RET receptor tyrosine kinase plays vital developmental and neuroprotective roles in metazoans. GDNF family ligands (GFLs) when bound to cognate GFRα co-receptors recognize and activate RET stimulating its cytoplasmic kinase function. The bipartite GFL-GFR complexes are recognized by the RET receptor tyrosine kinase (RTK) forming ternary RET-GFL-GFR complexes (Cacalano et al., 1998; Durbec et al., 1996; Jing et al., 1996; Treanor et al., 1996). RET has four consecutive cadherin-like domains (CLD(1-4)) and a membrane-proximal cysteine-rich domain (CRD) in its extracellular domain (RETECD) (Anders et al., 2001).

The zRGα1a cryo-EM map resembles a figure-of-eight with a molecular 2-fold centered at the crossover point. To enable building of a full structure into the map, we determined a crystal structure of zGDNFmat-zGFRα1a151-353 lacking domain D1 (referred to hereafter as zGFRα1aΔD1) at 2.2 Å (see the STAR Methods and Figure S5C). We then fitted crystal structures for zRET CLD(1-4) and zGDNFmat-zGFRα1aΔD1 into the symmetry-expanded map together with homology models for the zRETCRD and zGFRα1aD1. Some flexibility was apparent within the zGFRα1aΔ1-zGDNFmat. co-receptor-ligand complex itself and had been noted previously. The 2:2 complex X-ray crystal structure in the absence of RETECD has a distance of 127.9 Å between K325 of each GFRα1a protomer whereas in the presence of RETECD this distance increases to 131.3 Å.

> ENNCLNAAKACNLNDTCKKYRSAYISPCTSRVSTAEVCNKRKCHKALRQFFDKVPPKHSYGMLYCSCPLGDQSACSERRRQTIVPACSYEDKERPNCLTLQVSCKTNYICRSRLADFFTNCQPEPLSLSGCLKENYADCLLSYSGLIGTVMTPNYLRSPKISVSPFCDCSSSGNSKEECDRFTEFFTDNACLRNAIQAFGNGTGSEFLE;> QGRGCLLKEIHLNVTDLDLGYRTKEELIFRYCSGPCHDAETNYDKILNNLTHNKKLDKDTPSRTCCRPIAFDDDISFLDDSLEYHTLKKHSAKKCACV>[2x]GMTRTKLKLFVIGNSAISKRAIINLQSICSDPKLA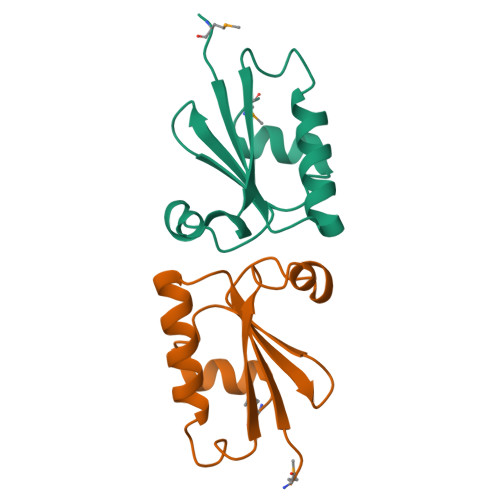DLCDIEVVDLCKNKGIAEQEKILATPILIKKEPLPERRIIGDLSDKQKVISALEMD> MPEIVDTCSLASPASVCRTKHLHLRCSVDFTRRTLTGTAALTVQSQEDNLRSLVLDTKDLTIEKVVINGQEVKYALGERQSYKGSPMEISLPIALSKNQEIVIEISFETSPKSSALQWLTPEQTSGKEHPYLFSQCQAIHCRAILPCQDTPSVKLTYTAEVSVPKELVALMSAIRDGETPDPEDPSRKIYKFIQKVPIPCYLIALVVGALESRQIGPRTLVWSEKEQVEKSAYEFSETESMLKIAEDLGGPYVWGQYDLLVLPPSFPYGGMENPCLTFVTPTLLAGDKSLSNVIAHEISHSWTGNLVTNKTWDHFWLNEGHTVYLERHICGRLFGEKFRHFNALGGWGELQNSVKTFGETHPFTKLVVDLTDIDPDVAYSSVPYEKGFALLFYLEQLLGGPEIFLGFLKAYVEKFSYKSITTDDWKDFLYSYFKDKVDVLNQVDWNAWLYSPGLPPIKPNYDMTLTNACIALSQRWITAKEDDLNSFNATDLKDLSSHQLNEFLAQTLQRAPLPLGHIKRMQEVYNFNAINNSEIRFRWLRLCIQSKWEDAIPLALKMATEQGRMKFTRPLFKDLAAFDKSHDQ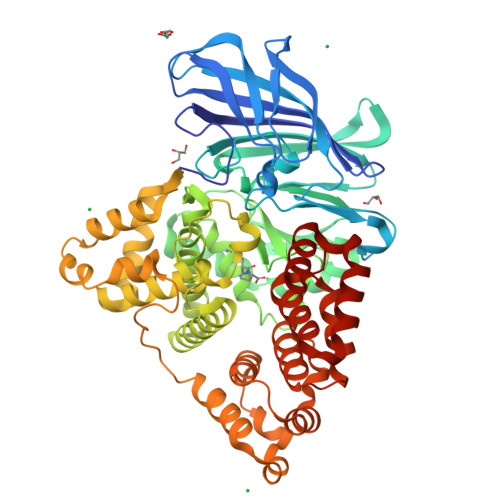AVRTYQEHKASMHPVTAMLVGKDLKVD>MNKTDLINAVAEQADLTKKEAGSAVDAVFESIQNSLAKGEKVQLIGFGNFEVRERAARKGRNPQTGKEID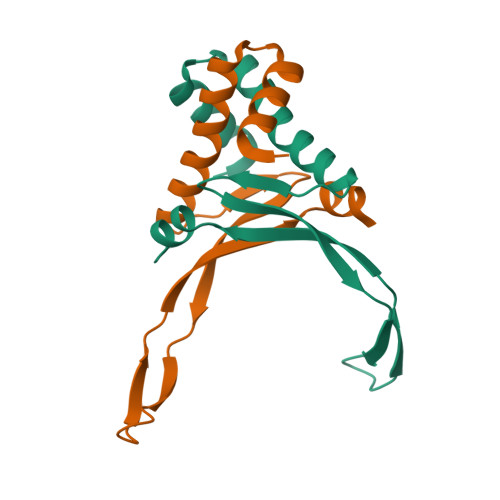IPASKVPAFKAGKALKDAVK[4x]> MASDAAAEPSSGVTHPPRYVIGYALAPKKQQSFIQPSLVAQAASRGMDLVPVDASQPLAEQGPFHLLIHKLYGDDWRAQLVAFAARHPAVPIVDPPHAIDRLHNRISMLQVVSELDHAADQDSTFGIPSQVVVYDAAALADFGLLAALRFPLIAKPLVADGTAKSHKMSLVYHREGLGKLRPPLVLQEFVNHGGVIFKVYVVGGHVTCVKRRSLPDVSPE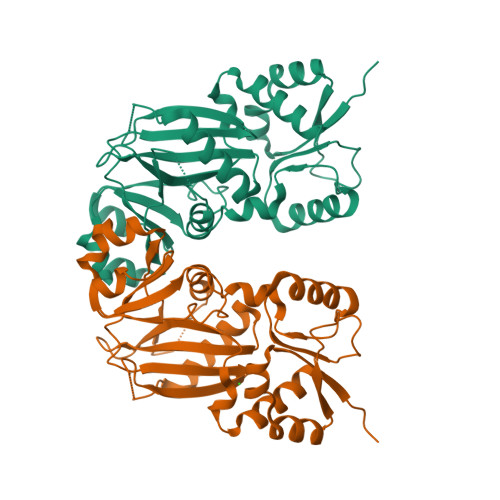DDASAQGSVSFSQVSNLPTERTAEEYYGEKSLEDAVVPPAAFINQIAGGLRRALGLQLFNFDMIRDVRAGDRYLVIDINYFPGYAKMPGYETVLTDFFWEMVHKDGVGNQQEEKGANHVVVK> MGHHHHHHRINHNIAALNTLNRLSSNNSASQKNMEKLSSGLRINRAGDDAAGLAISEKMRGQIRGLEMASKNSQDGISLIQTAEGALTETHAILQRVRE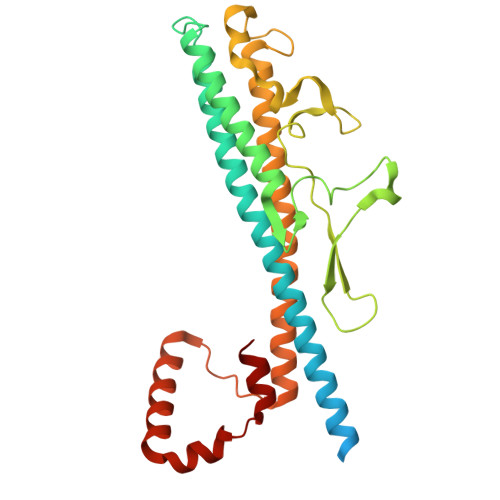LVVQAGNTGTQDKATDLQSIQDEISALTDEIDGISNRTEFNGKKLLDGTYKVDTATPANQKNLVFQIGANATQQISVNIEDMGADALGIKEADGSIAALHSVNDLDVTKFADNAADTADIGFDAQLKVVDEAINQVSSQRAKLGAVQNRLEHTINNLSASGENLTAAESRIRDVDMAKEMSEFTKNNILSQASQAMLAQANQQPQNVLQLLR> NTIQQLMMILNSASDQPSENLISYFNNCTVNPKESILKRVKDIGYIFKEKFAKAVGAGCVAIGSQRYKLGVRLYYRVMESMLKSEEERLSIQNFSKLLNDNIFHMSLLACALEVVMATYSRSTSQNLDSGTDLSFPWILNVLNLKAFDFYKVIESFIKAEGNLTREMIKHLERCEHRIMESLAWLSDSPLFDLIKQSKTREGKSTSLSLFYKKVYRLAYLRLNTLCERLLSEHPELEHIIWTLFQHTLQNEYELMRDRHL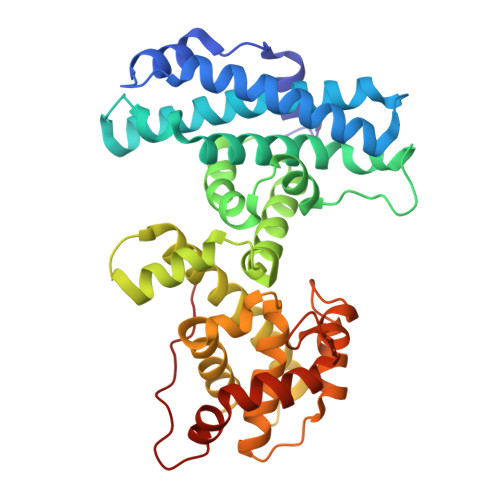DQIMMCSMYGICKVKNIDLKFKIIVTAYKDLPHAVQETFKRVLIKEEEYDSIIVFYNSVFMQRLKTNILQYASTRPPTLSPIPHI> GSSRAMGNEVAGVEDISVEIKPSSKRNSDARRTSRNVCSNEERKRRKYFHMLYLVCLMVHGFIRNEWINSKRLSRKLSNLVPEKVFELLHPQKDEELPLRSTRKLLDGLKKCMELWQKHWKITKKYDNEGLYMRTWKEIEMSANNKRKFKTLKRSDFLRAVSKGHGDPDISVQGFVAMLRACNVNARLIMSCQPPDFTNMKIDTSLNGNNAYKDMVKYPIFWCEVWDKFSKKWITVDPVNLKTIEQVRLHSKLAPKGVACCERNMLRYVIAYDRKYGCRDVTRRYAQWMNSKVRKRRITKDDFGEKWFRKVITALHHRKRTKIDDYEDQYFFQRDESEGIPDSVQDLKNHPYYVLEQDIKQTQIVKPGCKECGYLKVHGKVGKVLKVYAKRDIADLKSARQWYMNGRILKTGSRCKKVIKRTVGRPKGEAEEEDERLYSFEDTELYIPPLASASGEITKNTFGNIEVFAPTMIPGNCCLVENPVAIKAARFLGVEFAPAVTSFK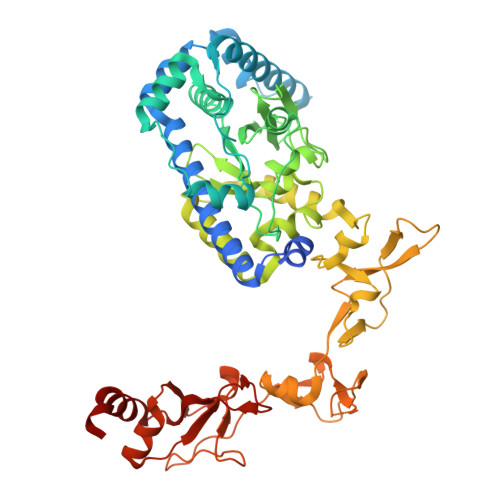FERGSTVKPVLSGIVVAKWLREAIETAIDGIEFI>AGGKVTSSTGIAPKRYVYYPGSEELGPDEIRVIACGTGMPTARRAQAAAAWVVELGNGDKFIVDIGSGSMANIQSLMIPANYLTKIFLTALHTDHWGDLVSMWAGGWTAGRTDPLEVWGPSGSREDMGTKYAVEHMLKAYNWDYMTRAVTINPRPGDINVHEFDYRALNEVVYQENGVTFRSWPCIHAGDGPVSFALE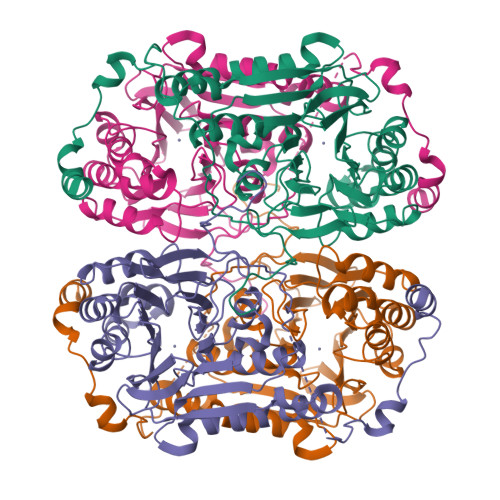WNGYKVVFGGDTAPNIWYPEYAKGADLAIHECWMTSDQMMTKYNQPAQLALRINLDFHTSAQSFGQIMNMVQPRHAVAYHFFNDDDTRYDIYTGVRENYAGPLSMATDMMVWNITRDAVTERMAVSPDHAWDVAGPSEDLAPDRNRASEYTQYILDGRLNVDEANAHWKQEFMG[8x]> SEKEKVEELAQRIREQLPDTELAREAQELADEARKSDDSEALKVVYLALRIVQQLPDTELAREALELAKEAVKSTDSEALKVVELALKIVQQLPDTELAKEALELAKEAVKSTDSEALKVVELALEIVQQLPDTELAKEALKLAKEAVKSTDSEALKVVYLALRIVQQLPDTELA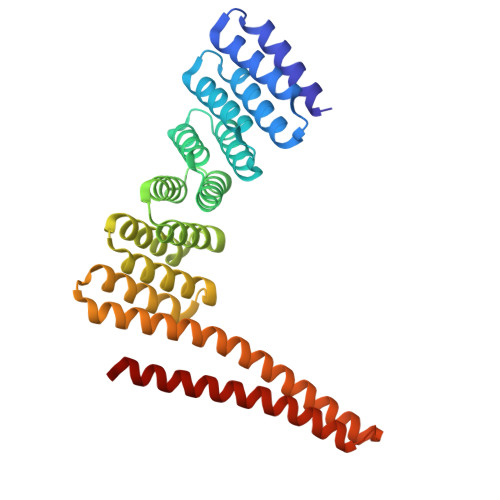REALELAKEAVKSTDSEQLEVVRLALEIVQLAPDTRLARAALKLAKEAVKSTDQEELKKVKAILRVASEVLKLEEEAKKSQEEVERLKQEVEKASKAGLDHEGDSRIFKKIHDVVTKQIKVILRLIAVYAELVAIIG> MTARAVRGTKDLFGKELRMHQRIVATARKVLEAAGALELVTPIFEETQVFEKGVGAATDIVRKEMFTFQDRGGRSLTLRPEGTAAMVRAYLEHGMKVWPQPVRLWMAGPMFRAERPQKGRYRQFHQVNYEALGSENPILDAEAVVLLYECLKELGLRRLKVKLSSVGDPEDRARYNAYLREVLSPHREALSEDSKERLEENPMRILDSKSERDQALLKELGVRPMLDFLGEEARAHLKEVERHLERLSVPYELEPALVRGLDYYVRTAFEVHHEEIGAQSALGGGGRYDGLSELLGGPRVPGVGFAFGVERVALALEAEGFGLPEEKGPDLYLIPLTEEAVAEAFYLAEALRPRLRAEYALAPRKPAKGLEEALKRGAAFAGFLGEDELRAGEVTLKRLAT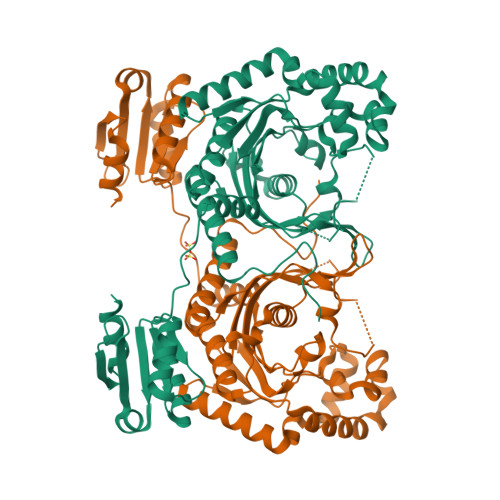GEQVRLSREEVPGYLLQALG> PTSKPTTTGKGCHIGRFKSLSPQELASFKKARDALEESLKLKNWSCSSPVFPGNWDLRLLQVRERPVALEAELALTLKVLEAAAGPALEDVLDQPLHTLHHILSQLQACIQPQPTAGPRPRGRLHHWLHRLQEAPKKESAGCLEASVTFNLFRLLTRDLKYVADGNLCLRTSTHPEST;> PGRPRLAPPQNVTLLSQNFSVYLTWLPGLGNPQDVTYFVAYQSSPTRRRWREVEECAGTKELLCSMMCLKKQDLYNKFKGRV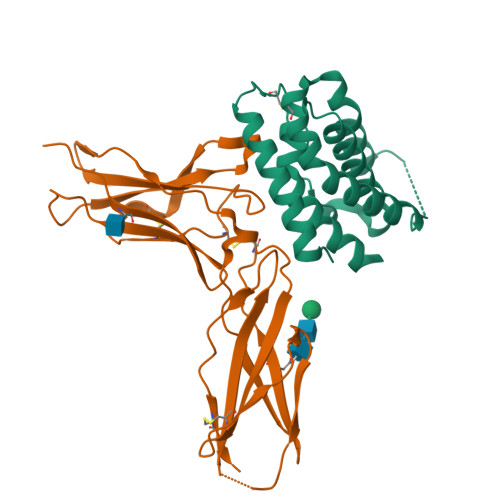RTVSPSSKSPWVESEYLDYLFEVEPAPPVLVLTQTEEILSANATYQLPPCMPPLDLKYEVAFWKEGAGNKTLFPVTPHGQPVQITLQPAASEHHCLSARTIYTFSVPKYSKFSKPTCFLLEVPEANASGSSGGSSGTSHHHHHH3-[(1E)-but-1-en-1-yl]-1-(2,2-diphosphonoethyl)pyridinium | C11 H18 N O6 P2 | 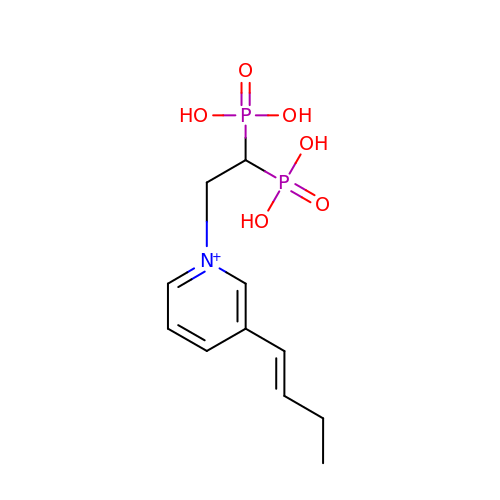QYIWBGUVYSKCTG-HWKANZROSA-O>HHHHHHMTIPDKIKAVYEKSTCLYTSNEVEAALDRMAIKIHETLQDKNPVIICVMVGGLVPLGNLLHRLDFPLEVDYVHATRYRGDLTGGDILWKVRPSSNLAGRTVLVVDDILDGGITLAAIINEIKAMGAAEVYSAVLVDKYRKRVPNGLQKADFVGLQVEDHYIFGYGMDYHEYLRNAPGIFIVHPDHEASK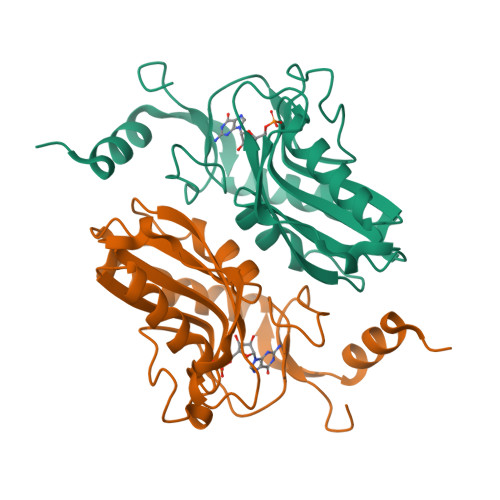[2x]>MMANRMILNETAWFGRGAVGALTDEVKRRGYQKALIVTDKTLVQCGVVAKVTDKMDAAGLAWAIYDGVVPNPTITVVKEGLGVFQNSGADYLI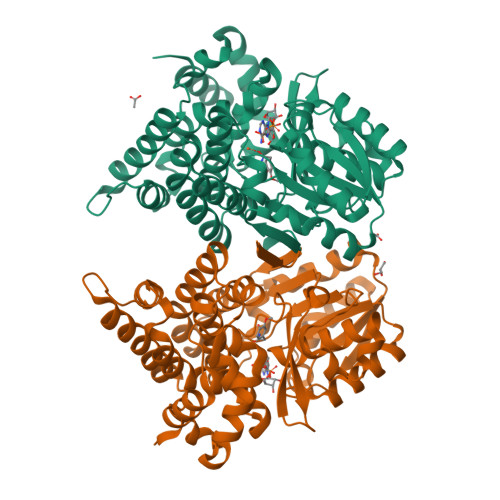AIGGGSPQDTCKAIGIISNNPEFADVRSLEGLSPTNKPSVPILAIPTTAGTAAEVTIGYVITDEEKRRKFVCVDPHDIPQVAFIDADMMDGMPPALKAATGVDALTHAIEGYITRGAWALTDALHIKAIEIIAGALRGSVAGDKDAGEEMALGQYVAGMGFSNVGVGLVHGMAHPLGAFYNTPHGVANAILLPHVMRYNADFTGEKYRDIARVMGVKVEGMSLEEARNAAVEAVFALNRDVGIPPHLRDVGVRKEDIPALAQAALDDVCTGGNPREATLEDIVELYHTAWTSHHHHH[2x]>[3x]MGSDKIHHHHHHENLYFQGMLLHLSTWQEVEAYLQQSKGIIFPIGSTEQHGPTGLIGTDAICAEAIAAGVGDATGAIVGPTINVGMALHHTAFPGTISLRPSTLIQVVRDYVTCLAKAGFSKFYFINGHGGNIATLKAAFSETYAHLEDLQIANAQQVQCQVANWFMCGSVYKLAKELYGDQEGSH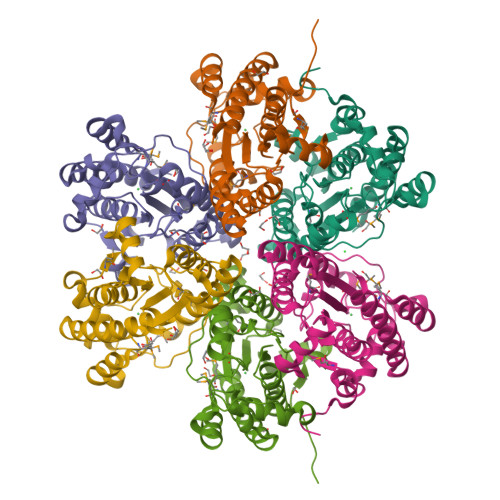ATPSEVALTQYVYPEAIKQAPLSPEVASGHRIYSAADFRVRYPDGRMGSNPGLATPEHGKQFYDLAVKELSNGYLEFVNAD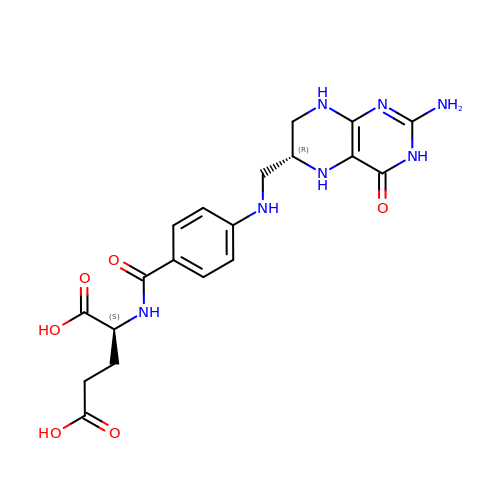N-[4-({[(6R)-2-amino-4-oxo-3,4,5,6,7,8-hexahydropteridin-6-yl]methyl}amino)benzoyl]-L-glutamic acid | C19 H23 N7 O6 | MSTNYGQPCMXVAQ-NEPJUHHUSA-N> MGSSHHHHHHSQDPENLYFQSMIPQFVIPLTNCLGQSYHFSSQPIPKGEHKKFDSEQSAKAFLDDFVPLRSSRVEELYHLLGQFPPNVPDEELTPELYAPVFAKALVNGSLYVASFPKTKKNATISSEPTPVPKQVKAKSKQNKAHTSSKTQAKNSASAKPLQTGSECHEKAGDPVSLVTGEEILTLNDVELPNGFVWSRTYRSSKASRNQGLGYGWRHAFQFELKEVTDEKHNVTSWEFISDSADEIEFEPVEHGSTSYQVYVGASCHFLNPNIRIVTLSSGDQYRFELVEDIWLLKQVRNGIFSTFQLRYSRNHRLIEVAHNKRPVLECQYDKQGRLVELLNAKTEQVLTTYIYDEQDDLVGATNDLGLTERYEYQDQHLIAKRVRPTGFTHYFEWSGEGSSAKCIRNFGDSGIYDYRFHYEGAKSSYSDSLDNEWTFIHDEQGHLLEKSSPTGRTWQWHYDHLGRKEKAVFPDNSTTQYQYNQQGQLISKLHSSGAQIQYGYDSLGKLVKTVSPDGDLEKAYYNSLGQRVWDIDALGCVTEYEYDKHGQVVKRESEDGKKSRWWWDKQQRLVAHEVDGTLLRYSYGATDLVNGIAYPDGCVAQISYDDYGRRTSIRYFNDEDKVGYSEEYAYDEFSRVAQIQTPEGVTSYQWGALAQQEAVIFPDGSHISYEYDQQRNLTKLVRSDGLAFEFWYDSEGLLSGTVGFDGLHSQFKYDSMGRIIRKDVADRTVLYSYDDAGFLQHIKAGNGKNIVENHFNYTLGGRLTLASNRHQTLQYQYSSFGHLTKRIQGQFEIGEEFNRVGQRVSQTLPDKTSFNFSYDTNGRLSEIRFSDDSLPKIEFQYDVMGRLSVTETESFRESKLYDGVGRLVEQQWSGREKKYIYNAQNRISSILDNTAGATHYQYDTLGYVTKVSEAGSTSTFESDSFGNPALADSKVMSDRIEAYAGVRYKYDQQGNQVKREGDGTVQKRVFDALSQ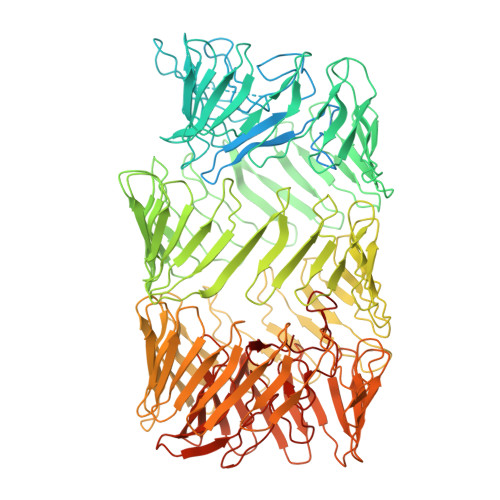LVEVHGDSSISHYEYDALGRRTKKITQNGITEFLWEGERLLGERTADGFRWYLYQPETYIPLAVLENGSIYLYECDQVGKPERLKDSAGNIVWSASYDVHGFASIDVEEVRNPLRFQGQYFDQETNLHYNLARYYDPKLGRFIQQDPISIAGGINHYQYAVNPIQWIDPTGF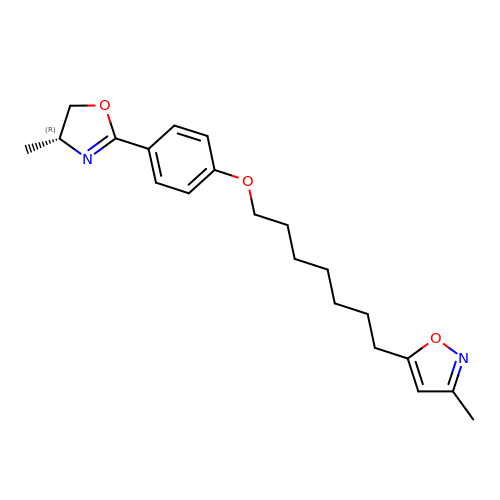5-(7-(5-HYDRO-4-METHYL-2-OXAZOLYL)PHENOXY)HEPTYL)-3-METHYL ISOXAZOLE | C21 H28 N2 O3 | NEAZMARKCJKUMF-QGZVFWFLSA-N> TIPKWWKEAVFYQVYPRSFKDTNGDGIGDINGIIEKLDYLKALGIDAIWINPHYDSPNTDNGYDIRDYRKIMKEYGTMEDFDRLISEMKKRNMRLMIDVVINHTSDQNEWFVKSKSSKDNPYRGYYFWKDAKEGQAPNNYPSFFGGSAWQKDEKTNQYYLHYFAKQQPDLNWDNPKVRQDLYAMLRFWLDKGVSGLRFDTVATYSKIPDFPNLTQQQLKNFAAEYTKGPNIHRYVNEMNKEVLSHYDIATAGEIFGVPLDQSIKFFDRRRDELNIAFTFDLIRLDRDSDQRWRRKDWKLSQFRQIIDNVDRTAGEYGWNAFFLDNHDNPRAVSHFGDDRPQWREPSAKALATLTLTQRATPFIYQGSELGMTNYPFKAIDEFDDIEVKGFWHDYVETGKVKADEFLQNVRLTSRDNSRT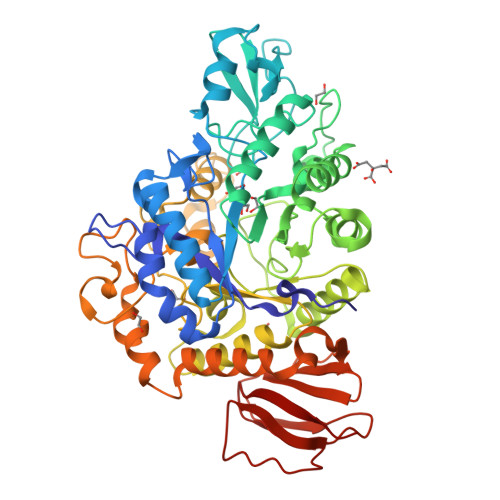PFQWDGSKNAGFTSGKPWFKVNPNYQEINAVSQVTQPDSVFNYYRQLIKIRHDIPALTYGTYTDLDPANDSVYAYTRSLGAEKYLVVVNFKEQMMRYKLPDNLSIEKVIIDSNSKNVVKKNDSLLELKPWQSGVYKLNQ> MGSSHHHHHHSQDPMAEPASVAAESLAGSRARAARTVLGQVVLPGEELLLPEQEDAEGPGGAVERPLSLNARACSRVRVVCGPGLRRCGDRLLVTKCGRLRHKEPGSGSGGGVYWVDSQQKRYVPVKGDHVIGIVTAKSGDIFKVDVGGSEPASLSYLSFEGATKRNRPNVQVGDLIYGQFVVANKDMEPEMVCIDSCG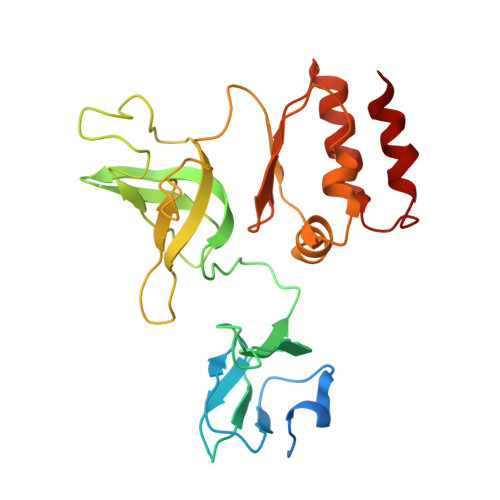RANGMGVIGQDGLLFKVTLGLIRKLLAPDCEIIQEVGKLYPLEIVFGMNGRIWVKAKTIQQTLILANILEACEHMTSDQRKQIFSRLAES> HHHHHHENLYFQHMSAPKDTIYHAKDAVQATKPDMR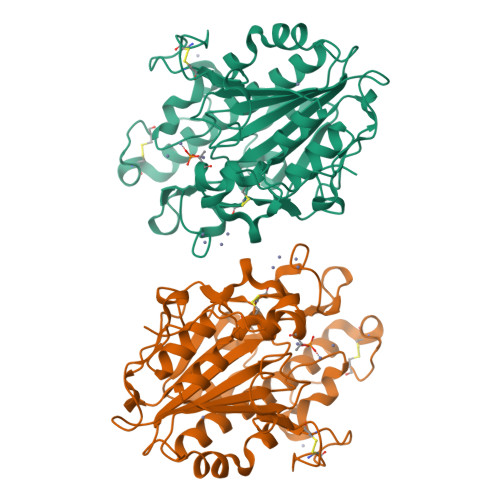KPRLVVFVVGETARADHVSFNGYERDTFPQLAKIDGVTNFSNVTSCGTSTAYSVPCMFSYLGADEYDVDTAKYQENVLDTLDRLGVSILWRDNNSDSKGVMDKLPKAQFADYKSATNNAICNTNPYNECRDVGMLVGLDDFVAANNGKDMLIMLHQMGNHGPAYFKRYDEKFAKFTPVCEGNELAKCEHQSLINAYDNALLATDDFIAQSIQWLQTHSNAYDVSMLYVSDHGESLGENGVYLHGMPNAFAPKEQRSVPAFFWTDKQTGITPMATDTVLTHDAITPTLLKLFDVTADKVKDRTAFIR>MNDSEFIQLADQLYQKIEEKIEESGADVDYDQNGSLLTLEFENHTKLIINRQQPLHQVWLATLENGHHYDYNNGKWIDDRSGDE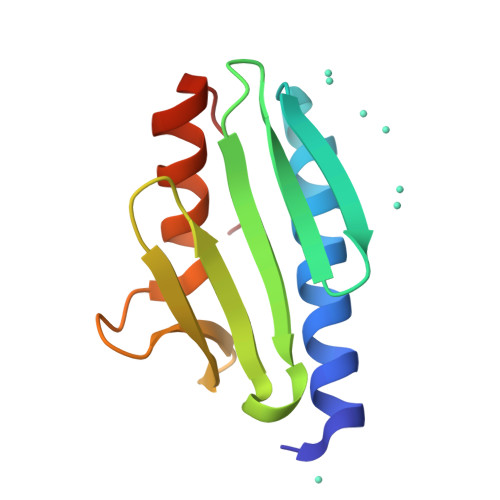FLTFLSAAIFKQSKETVDFTE[2x]The respective glycosyltransferases are important virulence factors such as the Clostridioides difficile toxins A and B. Here, we describe two glycosyltransferases of Yersinia species that have a high sequence identity: YeGT from the zoonotic pathogen Yersinia enterocolitica and YkGT from the murine pathogen Yersinia kristensenii. We show that both modify Rho family proteins by attachment of GlcNAc at tyrosine residues (Tyr-34 in RhoA). sYeGT has a cone-shaped structure comprised of a globular domain with a Rossmann-like fold on top of a three-helix bundle. The catalytically active domain is the Rossmann-like fold domain, which features a 6-stranded antiparallel β-sheet flanked by 7 α-helices.

In order to characterize the mechanism of operation of these proteins and to shed light onto their architecture, we initiated crystallization trials with different constructs. sYeGT was crystallized in the absence of ligands and in the presence of UDP-GlcNAc and manganese chloride. Interestingly, in the absence of ligands, sYeGT crystals belonging to space group P43212 appeared rapidly and diffracted X-rays up to 2.3-Å resolution while in the presence of UDP-GlcNAc, P21 crystals were visible only after 8 weeks but diffracted better, with a resolution up to 1.12 Å. After accurate determination of twinning parameters, the phase problem of the ligand bound structure was solved by molecular replacement and refined to final R and Rfree values of 15.3 and 16.9, respectively. This structure was consequently used to support molecular replacement and model building of the ligand free structure, which was refined to final R and Rfree values of 20.4 and 24.5, respectively. The ligand-free structure features four molecules in the asymmetric unit. All protomers show clear features in the electron density map for residues 258 to 267, so that they could be included in the structure. Similar to the ligand-bound structure, the C-terminal residues were not resolved and not included in the final structure. Superimposition of the ligand-free and ligand bound sYeGT structures showed no major conformational change upon nucleotide binding. Residues 257 to 267, which are resolved in the ligand-free structure only, form a loop that connects two helices of the 3-helix bundle. At the C terminus, the last resolved residues (294–301) are covering the empty nucleotide-binding site in the ligand free structure, while they are pointing outward in the UDP-bound sYeGT structure. In the ligand free structure, Asp-298 stabilizes the covering position of the C terminus over the unoccupied nucleotide binding side, as it forms a salt bridge with Lys-53, a residue located close to the uridine base binding site.

>[4x]GSMQYFAQIVNREENKWPSEPINKYIHMIWIGPKNISDKNIRLSLQTAQKNPDYSTTIIYDSGISGYEAARNFMSEKFKASKITLVDIRNKGYFHQLQQEPSFTYYEEVIRNKKFAQASDILRLLVLKYEGGIYKDIDDIQIKGFGSLAFPKGIGVMREYVPEAGKSAAFPNSPIAATKNNPVVNKTLELAVENYRHGEKNVLKLAGPDVFTKALYQEIPGMCSQVLGTQLEQFELAKRQALKMPLEKPKSFIDEQLTLQEKAKISRPYKAIRGLSEYVCNGADHSWATDMLGSSTKMY> RQGCEARRAHEHLIRLLLEQGKCPEDGWDESTLELFLHELAVMDSNNFLGNCGVGEREGRVASALVARRHYRFIHGIGRSGDISAVQPKAAGSSLLNKITNSLVLNVIKLAGVHSVASCFVVPMATGMSLTLC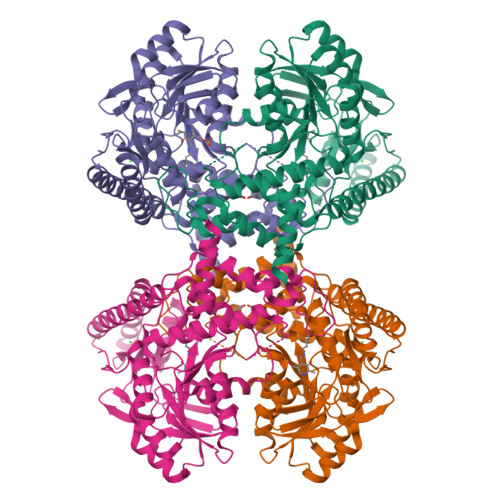FLTLRHKRPKAKYIIWPRIDQKSCFKSMVTAGFEPVVIENVLEGDELRTDLKAVEAKIQELGPEHILCLHSTTACFAPRVPDRLEELAVICANYDIPHVVNNAYGLQSSKCMHLIQQGARVGRIDAFVQSLDKNFMVPVGGAIIAGFNEPFIQDISKMYPGRASASPSLDVLITLLSLGCSGYRKLLKERKEMFVYLSTQLKKLAEAHNERLLQTPHNPISLAMTLKTIDGHHDKAVTQLGSMLFTRQVSGARAVPLGNVQTVSGHTFRGFMSHADNYPCAYLNAAAAIGMKMQDVDLFIKRLDKCLNIVRKEQTRA> AVEPKEDTITVTAAPAPQESAWGPAATIAARQSATGTKTDTPIQKVPQSISVVTAEEMALHQPKSVKEALSYTPGVSVGTRGASNTYDHLIIRGFAAEGQSQNNYLNGLKLQGNFYNDAVIDPYMLERAEIMRGPVSVLYGKSSPGGLLNMVSKRPTTEPLKEVQFKAGTDSLFQTGFDFSDSLDDDGVYSYRLTGLARSANAQQKGSEEQRYAIAPAFTWRPDDKTNFTFLSYFQNEPETGYYGWLPKEGTVEPLPNGKRLPTDFNEGAKNNTYSRNEKMVGYSFDHEFNDTFTVRQNLRFAENKTSQNSVYGYGVCSDPANAYSKQCAALAPADKGHYLARKYVVDDEKLQNFSVDTQLQSKFATGDIDHTLLTGVDFMRMRNDINAWFGYDDSVPLLNLYNPVNTDFDFNAKDPANSGPYRILNKQKQTGVYVQDQAQWDKVLVTLGGRYDWADQESLNRVAGTTDKRDDKQFTWRGGVNYLFDNGVTPYFSYSESFEPSSQVGKDGNIFAPSKGKQYEVGVKYVPEDRPIVVTGAVYNLTKTNNLMADPEGSFFSVEGGEIRARGVEIEAKRPLSASVNVVGSYTYTDAEYTTDTTYKGNTPAQVPKHMASLWADYTFFDGPLSGLTLGTGGRYTGSSYGDPANSFKVGSYTVVDALVRYDLARVGMAGSNVALHVNNLFDREYVAS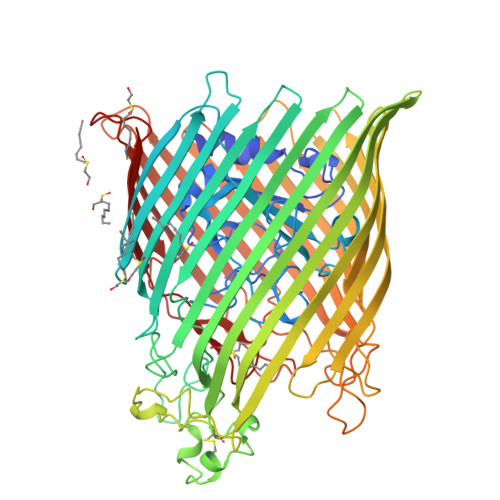CFNTYGCFWGAERQVVATATFRF>[2x]YAEHKSHRGEYSVCDSESLWVTDKSSAIDIRGHQVTVLGEIKTGNSP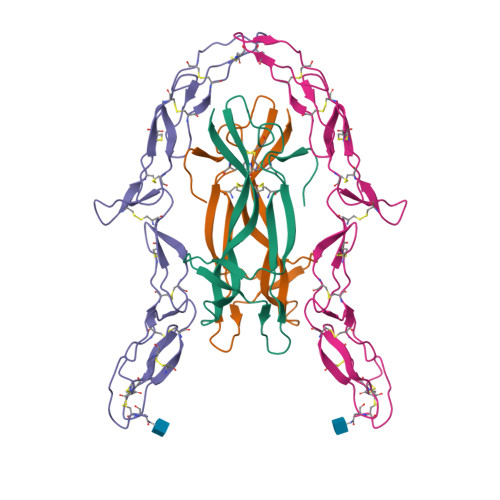VKQYFYETRCKEARPVKNGCRGIDDKHWNSQCKTSQTYVRALTSENNKLVGWRWIRIDTSCVCALSRKIGRT;>KETCSTGLYTHSGECCKACNLGEGVAQPCGANQTVCEPCLDSVTFSDVVSATEPCKPCTECLGLQSMSAPCVEADDAVCRCAYGYYQDEETGHCEACSVCEVGSGLVFSCQDKQNTVCEECPEGTYSDEANHVDPCLPCTVCEDTERQLRECTPWADAECEHHHHHH[2x]> TTHYSVADRWGNAVSVTYTINASYGSAASIDGAGFLLNNEMDDFSIKPGNPNLYGLVGGDANAIEANKRPLSSMSPTIVLKNNKVFLVVGSPGGSRIITTVLQVISNVIDYNMNISEAVSAPRFHMQWLPDELRIEKFGMPADVKDNLTKM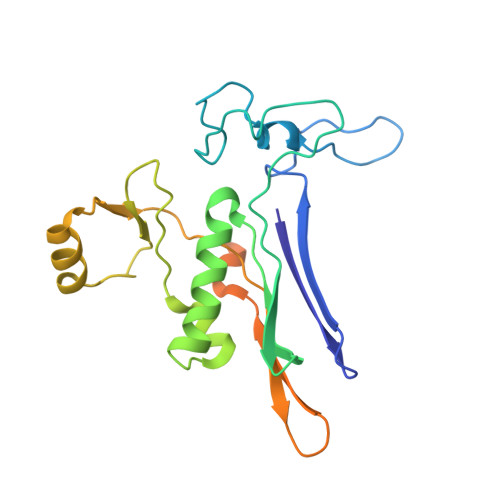GYQIVTKPVMGDVNAIQVLPKTKGSVFYGSTDPRKEFGTGSKLAAAQLYTRASQPELAPEDPEDLEHHHHHHHH>MKHHHHHHHHHHSAGLEVLFQGPYVQAFDSLLANPVAEYLKMSKEIGGDVQKHAEMVHTGLKLERALLATASQCQQP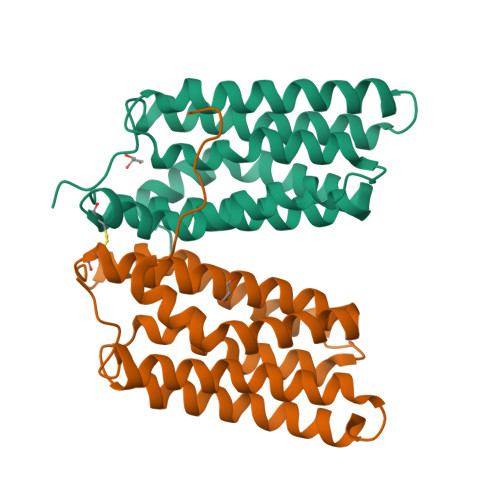AGNKLSDLLAPISEQIQEVITFREKNRGSKFFNHLSAVSESIQALGWVALAAKPGPFVKEMNDAAMFYTNRVLKEYRDVDKKHVDWVRAYLSIWTELQAYIKEFHTTGLAWSKTGPVAKEL[4x]> SNAQVQVGAPEEEEEEEEDAGLVAEAEAVAAGWMLDFLCLSLCRAFRDGRSEDFRRTRNSAEAIIHGLSSLTACQLRTIYICQFLTRIAAGKTLDAQFENDERITPLESALMIWGSIEKEHDKLHEEIQNLIKIQAIAVCMENGNFKEAEEVFERIFGDPNSHMPFKSKLLMIISQKDTFHSFFQHFSYNHMMEKIKSYVNYVLSEKSSTFLMKAAAKVVESKR

TRF1 is a subunit of the shelterin complex that binds to and protects the linear ends of chromosomes known as telomeres. TRF1 binds to double-stranded telomeric repeats and mediates telomere protection, replication and extension. It is recruited to shelterin through a domain:peptide interaction between its TRF homology (TRFH) domain, also responsible for dimerisation of TRF1 (TRF1TRFH), and a short linear motif of TIN2, known as its TRFH-binding motif or TBM (TIN2TBM). Here, we report the discovery of a series of fragment hits that bind at the interface between the TRFH domain of TRF1 (TRF1TRFH) and a peptide of TIN2 (TIN2TBM), an interaction essential for the recruitment of TRF1 to shelterin, using X-ray crystallography (XChem) and ligand-observed NMR (LO-NMR) fragment screening.

To find a different crystal form of TRF1TRFH, we carried out a series of commercially available crystallisation screens and identified conditions that generated crystals in the P41212 space group, different from the original P3121 crystal system. An initial inspection of the TIN2TBM site showed that the closest neighbouring TRF1TRFH molecule in this new crystal was further away than in the previous crystal system, this time exposing both the TIN2 leucine and phenylalanine binding pockets to the solvent. Furthermore, the loop region adjacent to the leucine pocket that typically accommodates three arginine residues of TIN2 was well-resolved and closely resembled that of the published TRF1:TIN2 co-crystal structure; this was in contrast to the previous crystal system, in which F142 formed a cation-pi interaction with the sidechain of R131. In light of this, we carried out a second XChem fragment screen against the new crystal system of TRF1TRFH. PanDDA analysis of the 981 processable datasets resulted in 50 hits being identified across different sites of the protein, 28 of which were found in the TIN2TBM binding site. After refinement of the 28 PanDDA hits, 19 could be confidently assigned in the conventional electron density maps. However, unlike the hits obtained from the P3121 XChem screen, the hits from the P41212 XChem screen spanned a larger surface area of the TIN2TBM binding site, and most did not appear to form any interactions with TRF1TRFH molecules from neighbouring asymmetric units. This diversity of hit matter covering the leucine pocket and the phenylalanine pocket of the TIN2TBM peptide will provide a firm starting point for efforts aimed at linking and merging hits. Interestingly, several fragment hits originating from our second XChem screen possess alternative groups to the sulfonic acid that interact with R131 and R102, which opens up opportunities to link and merge hit matter found across the TIN2 leucine and phenylalanine binding pockets.> MAAFTPQWNDWCPGCGNFGILNAEQQAIVELGVDTKNVVVVSGIGCSGKIPHFFRTPISGVHTLHGRAIAFATGIKLSNPDLVVIVNGGDGDLLGIGAGHFVAAGRRNVDMVVILHDNGVYGLTKGQASPTLKRGEKPKSLPRPNINDAVNPIALAISSGYTFVARGYAYDVKHLKELIKSAIKHKGLALIDVLQPCPTYNDINTKEWYDKRIYKLDTLPDWDPVVKKPEEVNEKIKRAIDKSLEWGDRIPIGIFYQNELVPSYEERIKANSPAYLDYTPAKQLIEKEGKLTTIIDPLLKEREV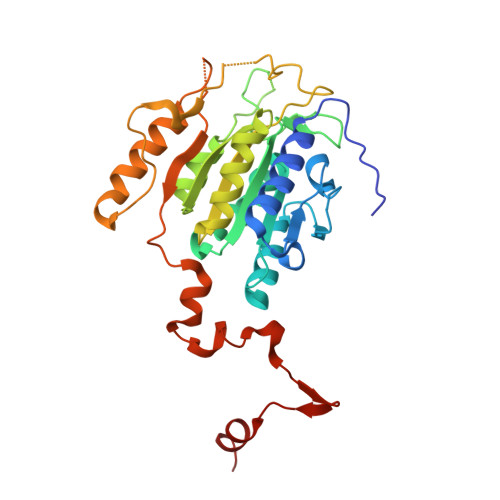D> MAVVEFAGSAFEVDEDGFLNAFDDWCPEWVKYAKGSEGIGAGSADHQKIIDF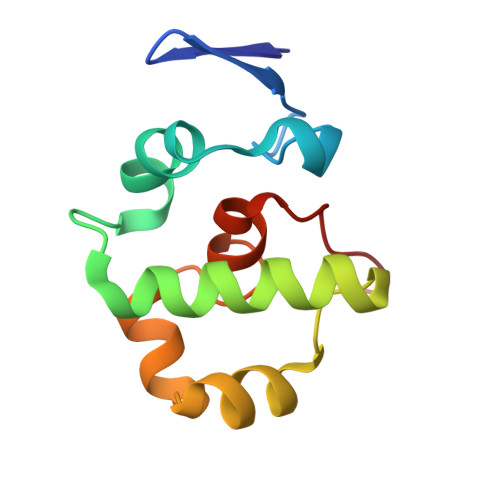LQDYYKANGIAPMVRILSKNTGFALKEIYELFPSGPGKGACKMAGLPKPTGCV(Z)-L-Arabinonhydroximo-1,4-lactone 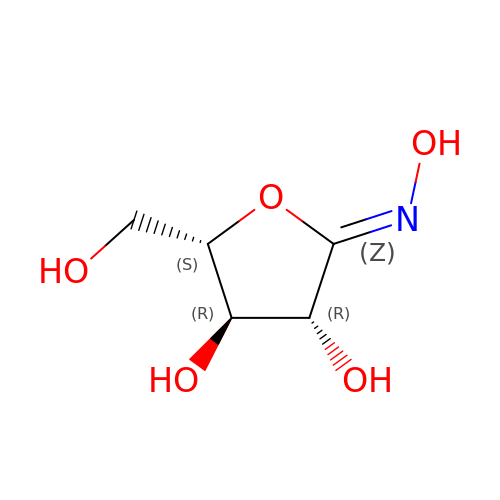| C5 H9 N O5 | AVHYWFZJLLOYOD-XXXIWBGBSA-N>[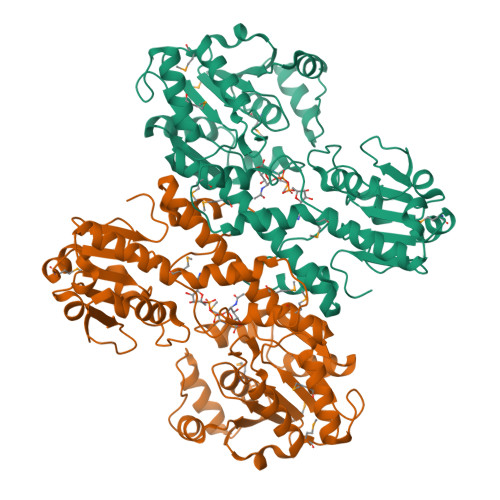2x]MRIAVLGLGYIGLPTAIMFASSGYDVVGYDIRSEVIKKINSGVAHIIEPEIDRRLKEVLSLGKLKVTDRVEDLKGSNVFIICVQTPLSGDDPDLSYLERAIRTVAEVMDRGALVIIESTIPPGTTEKMARLLENLTGLREGVDFYVAHAPERVMPGRIFKELVYNSRIIGGVSEKAANLAEKLYRSFVKGRIFLTNATTAEMVKLMENTFRDVNIALANEFALLAHQYGVNVYEAIELANTHPRVKIHTPGIGVGGHCLPKDPYLLLSNAKEDFGLIRIARRINERMPAFAAGLLFEALEKANIKPSEAIIAVLGLAYKGGTDDTRNSPALKFVEIIRNSVKEVRTYDPYVRGTHDSLEKVVEGADAIVIATDHPEFKSVNWESIGKSMRHKIIIDGRNIIKEPPVGFIFRGIGRGDV(1S,2S,3R,4S,6R)-4,6-diamino-3-{[(2S,3R)-3-amino-6-(fluoromethyl)-3,4-dihydro-2H-pyran-2-yl]oxy}-2-hydroxycyclohexyl 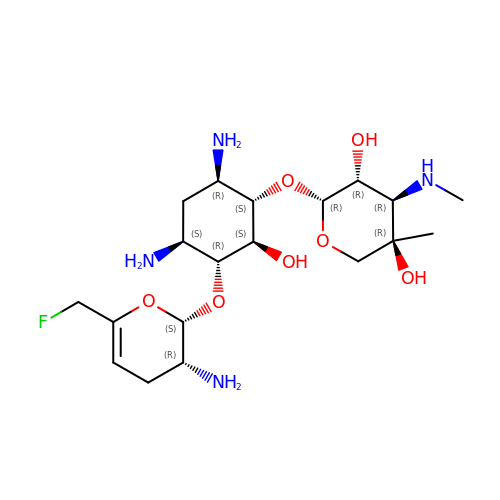3-deoxy-4-C-methyl-3-(methylamino)-beta-L-arabinopyranoside | C19 H35 F N4 O7 | WYTHUXIFAFNYLB-YFMIWBNJSA-N> MNFNVSLMEKLKWKIKCIENKFLNYRLTTNETVVAETEYGKVKGVKRLTVYDDSYYSFEGIPYAQPPVGELRFKAPQRPTPWAGVRDCCNHKDKSVQVDFITGKVCGSEDCLYLSVYTNNLNPETKRPVLVYIHGGDFIIG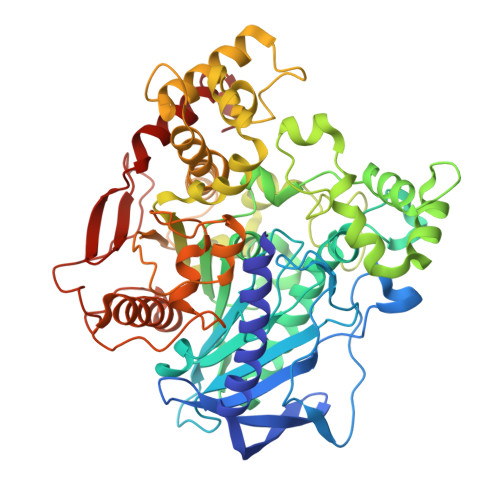ENHRDMYGPDYFIKKDVVLINIQYRLGALGFLSLNSEDLNVPGNAGLKDQVMALRWIKNNCANFGGNPDNITVFGESAGAASTHYMMLTEQTRGLFHRGILMSGNAICPWANTQCQHRAFTLAKLAGYKGEDNDKDVLEFLMKAKPQDLIKLEEKVLTLEERTNKVMFPFGPTVEPYQTADCVLPKHPREMVKTAWGNSIPTMMGNTSYEGLFFTSILKQMPLLVKELETCVNFVPSELADAERTAPETLEMGAKIKKAHVTGETPTADNFMDLCSHFYFWFPMHRLLQLRFNHTSGTPVYLYRFDFDSEDLINPYRIMRSGRGVKGVSHTDELTYFFWNQLAKRMPKESREYKTIERMTGIWTQFATTGNPYSNEIEGMENVSWDPIEKSDEVYKCLNISDELKMIDVPEMGKIKQWESMFEKHRDLF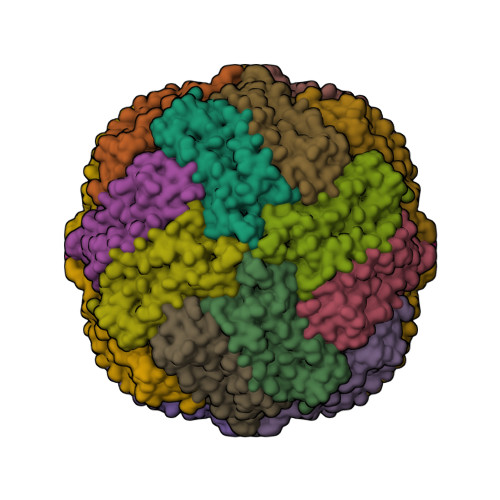> SSQIRQNYSTEVEAAVNRLVNLYLRASYTYLSLGFYFDRDDVALCGVCHFFCELAEEKREGAERLLKMQNQRGGRALFQDLQKPSQDEWGTTLDAMKAAIVLEKSLNQALLDLHALGSAQADPHLCDFLESHFLDEEVKLIKKMGDHLTNIQRLVGSQAGLGEYLFERLTLKHD> MSLRWQWRIYEEPLQEPLTTAQGVWRSRSGIYLRLEDEQGQVGYGEIAPLPGWGSETLNADIALCQQLPGHLTPEIMATIPEALPAAQFGFATAWQSVGRLPYRVRPWPICALLGSGQAALEQWQQSWQRGQTTFKWKVGVMSPEEEQAILKALLAALPPGAKLRLDANGSWDRATANRWFAWLDRHGNGKIEYVEQPLPPDQWQALLSLAQTVTTAIALDESVVSAAEVQRWVDRGWPGFFVIK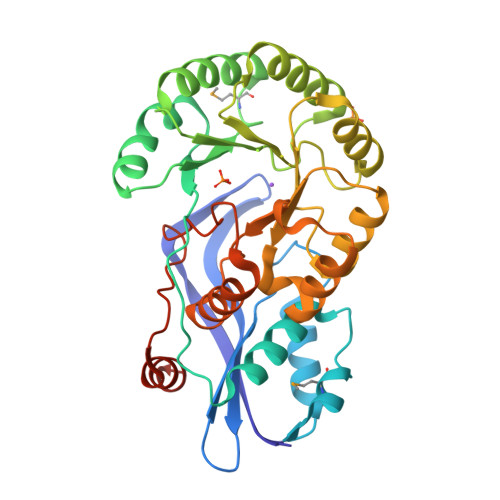TALFGDPDSLSLLLRRGLEPQRLVFSSALEGAIARTAIFHLLETWQPCHALGFGVDRWRSAPLLTTLTAYERLWERLDQEGHHHHHH>MACGSSAVIKTDAGSVTQDELYEAMKTTYGNEVVQQLTFKKILEDKYTVTEKEVNAEYKKYEEQYGDSFESTLSSNNLTKTSFKENLEYNLLVQKATEANMDVSESKLKAYYKTWEPDITVRHILVDDEATAKEIQTKLKNGEKFTDLAKEYSTDTATSTNGGLLDPFGPGEMDETFEKAAYALENKDDVSGIVKSTYGYHLIQLVKKTEKGTYAKEKANVKAAYIKSQLTSENMTAALKKELKAANIDIKDSDLKDAFADYTSTSSTSSTTTSNR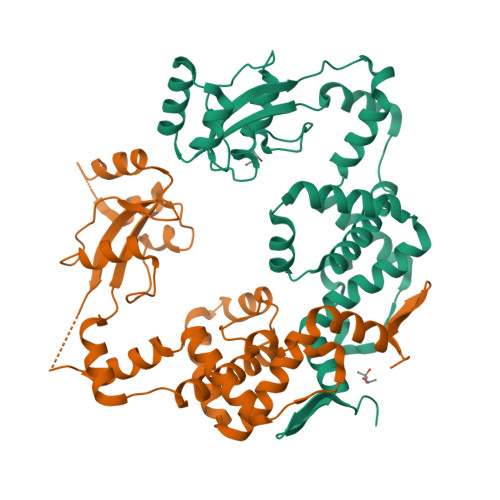SHHHHHH[2x]>[4x]MRDLKGIFSALLVSFNEDGTINEKGLRQIIRHNIDKMKVDGLYVGGSTGENFMLSTEEKKEIFRIAKDEAKD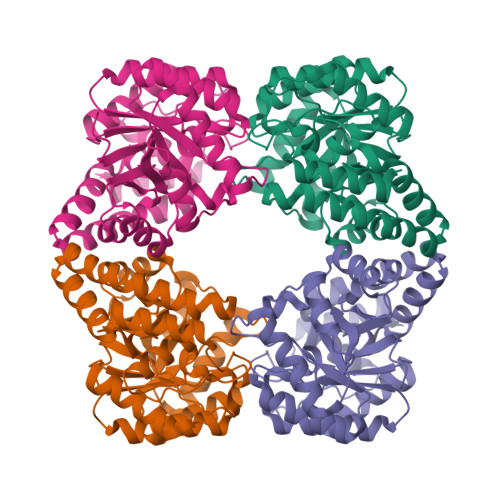QIALIAQVGSVNLKEAVELGKYATELGYDCLSAVTPFYYKFSFPEIKHYYDTIIAETGSNMIVYSIPFLTGVNMGIEQFGELYKNPKVLGVKFTAGDFYLLERLKKAYPNHLIWAGFDEMMLPAASLGVDGAIGSTFNVNGVRARQIFELTKAGKLKEALEIQHVTNDLIEGILANGLYLTIKELLKLEGVDAGYCREPMTSKATAEQVAKAKDLKAKFLS> MSLSFCGNNISSYNIYHGVLQNPCFVDALNLVPHVFLLFITFPILFIGWGSQSSKVQIHHNTWLHFPGHNLRWILTFALLFVHVCEIAEGIVSDSQRASRHLHLFMPAVMGFVATTTSIVYYHNIETSNFPKLLLALFLYWVMAFITKTIKLVKYWQLGWGMSDLRFCITGVMVILNGLLMAVEINVIRVRRYVFFMNPQKVKPPEDLQDLGVRFLQPFVNLLSKATYWWMNTLIISAHRKPIDLKAIGKLPIAMRAVTNYVCLKEAYEEQKKKAADHPNRTPSIWLAMYRAFGRPILLSSTFRYLADLLGFAGPLCI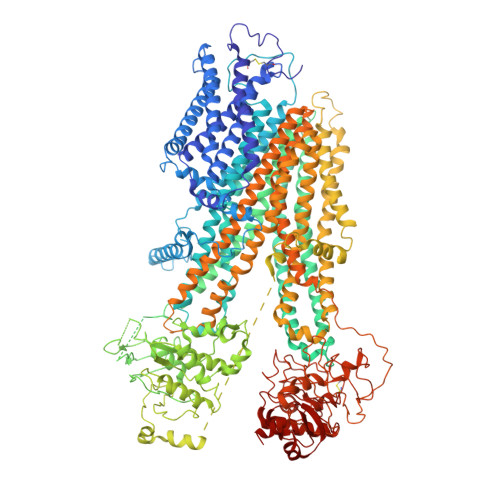SGIVQRVNEPKNNTTRFSETLSSKEFLENAHVLAVLLFLALILQRTFLQASYYVTIETGINLRGALLAMIYNKILRLSTSNLSMGEMTLGQINNLVAIETNQLMWFLFLCPNLWAMPVQIIMGVILLYNLLGSSALVGAAVIVLLAPIQYFIATKLAEAQKSTLDYSTERLKKTNEILKGIKLLKLYAWEHIFCKSVEETRMKELSSLKTFALYTSLSIFMNAAIPIAAVLATFVTHAYASGNNLKPAEAFASLSLFHILVTPLFLLSTVVRFAVKAIISVQKLNEFLLSDEIGEDSWRTGEGTLPFESCKKHTGVQSKPINRKQPGRYHLDNYEQARRLRPAETEDVAIKVTNGYFSWGSGLATLSNIDIRIPTGQLTMIVGQVGCGKSSLLLAILGEMQTLEGKVYWNNVNESEPSFEATRSRSRYSVAYAAQKPWLLNATVEENITFGSSFNRQRYKAVTDACSLQPDIDLLPFGDQTEIGERGINLSGGQRQRICVARALYQNTNIVFLDDPFSALDIHLSDHLMQEGILKFLQDDKRTVVLVTHKLQYLTHADWIIAMKDGSVLREGTLKDIQTKDVELYEHWKTLMNRQDQELEKDMEADQTTLERKTLRRAMYSREAKAQMEDEDEEEEEEEDEDDNMSTVMRLRTKMPWKTCWWYLTSGGFFLLFLMIFSKLLKHSVIVAIDYWLATWTSEYSINDPGKADQTFYVAGFSILCGAGIFLCLVTSLTVEWMGLTAAKNLHHNLLNKIILGPIRFFDTTPLGLILNRFSADTNIIDQHIPPTLESLTRSTLLCLSAIGMISYATPVFLIALAPLGVAFYFIQKYFRVASKDLQELDDSTQLPLLCHFSETAEGLTTIRAFRHETRFKQRMLELTDTNNIAYLFLSAANRWLEVRTDYLGACIVLTASIASISGSSNSGLVGLGLLYALTITNYLNWVVRNLADLEVQMGAVKKVNSFLTMESENYEGTMDPSQVPEHWPQEGEIKIHDLCVRYENNLKPVLKHVKAYIKPGQKVGICGRTGSGKSSLSLAFFRMVDIFDGKIVIDGIDISKLPLHTLRSRLSIILQDPILFSGSIRFNLDPECKCTDDRLWEALEIAQLKNMVKSLPGGLDATVTEGGENFSVGQRQLFCLARAFVRKSSILIMDEATASIDMATENILQKVVMTAFADRTVVTIAHRVHTILTADLVIVMKRGNILEYDTPESLLAQEDGVFASFVRADM>MSLSINSREVLAEKVKNAVNNQPVTDMHTHLFSPNFGEILLWDIDELLTYHYLVAEVMRWTDVSIEAFWAMSKREQADLIWEELFIKRSPVSEACRGVLTCLQGLGLDPATRDLQVYREYFAKKTSEEQVDTVLQLANVSDVVMTNDPFDDNERISWLEGKQPDSRFHAALRLDPLLNEYEQTKHRLRDWGYKVNDEWNEGSIQEVKRFLTDWIERMDPVYMAVSLPPTFSFPEESNRGRIIRDCLLPVAEKHNIPFAMMIGVKKRVHPALGDAGDFVGKASMDGVEHLLREYPNNKFLVTMLSRENQHELVVLA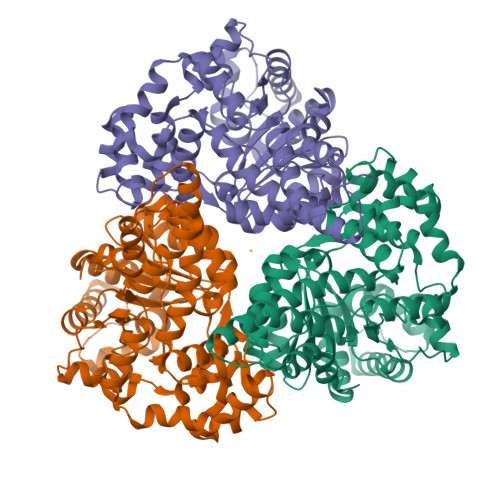RKFSNLMIFGCWWFMNNPEIINEMTRMRMEMLGTSFIPQHSDARVLEQLIYKWHHSKSIIAEVLIDKYDDILQAGWEVTEEEIKRDVADLFSRNFWRFVGRNDHVTSVKVEQQTEGHHHHHH[12x]1-(3-{[(3Z)-2-oxo-3-(1H-pyrrol-2-ylmethylidene)-2,3-dihydro-1H-indol-6-yl]amino}phenyl)-3-[3-(trifluoromethyl)phenyl]urea 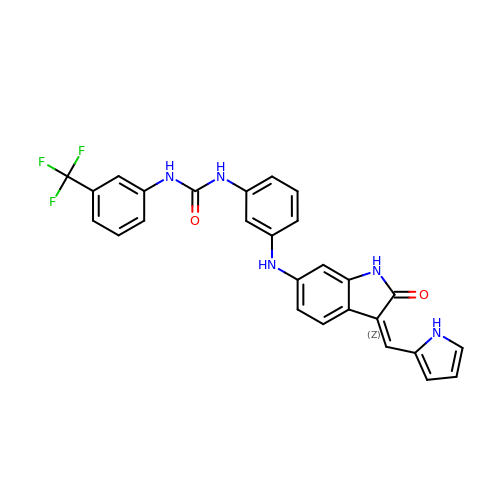| C27 H20 F3 N5 O2 | JCRUDKWPDBIGME-UCQKPKSFSA-N> SDK;> SNAGGSSPITGLVYDQRMMLHHNMWDSHHPELPQRISRIFSRHEELRLLSRCHRIPARLATEEELALCHSSKHISIIKSSEHMKPRDLNRLGDEYNSIFISNESYTCALLAAGSCFNSAQAILTGQVRNAVAIVRPPGHHAE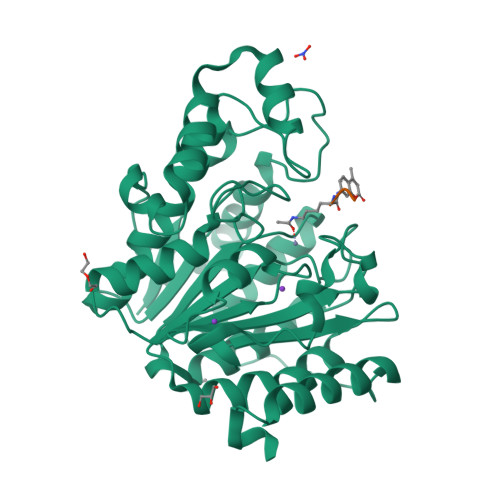KDTACGFCFFNTAALTARYAQSITRESLRVLIVDWDVHHGNGTQHIFEEDDSVLYISLHRYEDGAFFPNSEDANYDKVGLGKGRGYNVNIPWNGGKMGDPEYMAAFHHLVMPIAREFAPELVLVSAGFDAARGDPLGGFQVTPEGYAHLTHQLMSLAAGRVLIILEGGFNLTSISESMSMCTSMLLGDSPPSLDHLTPLKTSATVSINNVLRAHAPFWSSLR1-(morpholin-4-yl)-4-phenylbutan-1-one | C14 H19 N O2 | 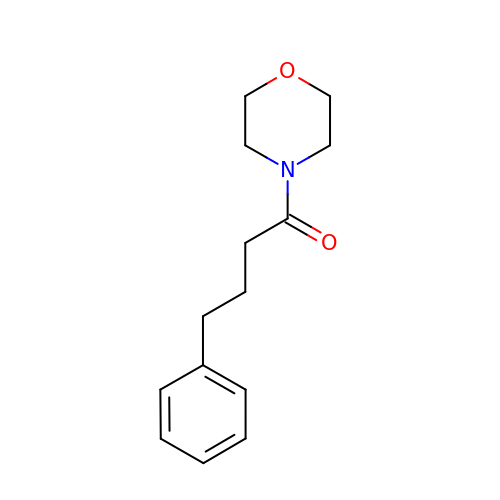VCWRKWJSYZSPEJ-UHFFFAOYSA-N>MNIHGFDLGSRYMDLKPLGCGGNGLVFSAVDNDCDKRVAIKKIVLTDPQSVKHALREIKIIRRLDHDNIVKVFEILGPS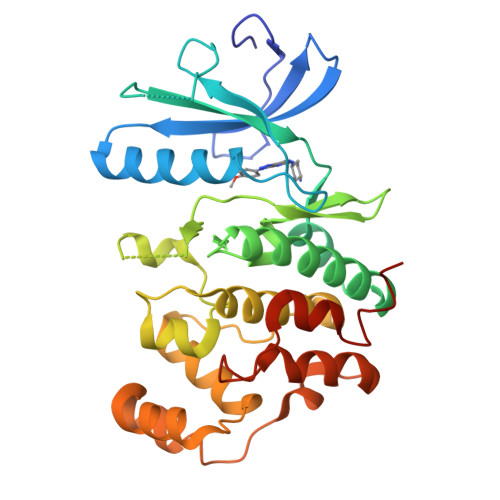GSQLTDDVGSLTELNSVYIVQEYMETDLANVLEQGPLLEEHARLFMYQLLRGLKYIHSANVLHRDLKPANLFINTEDLVLKIGDFGLARIMDPHYSHKGHLSEGLVTKWYRSPRLLLSPNNYTKAIDMWAAGCIFAEMLTGKTLFAGAHELEQMQLILESIPVVHEEDRQELLSVIPVYIRNDMTEPHKPLTQLLPGISREAVDFLEQILTFSPMDRLTAEEALSHPYMSIYSFPMDEPI[2x]>GMQSAYSFLPQVIAHRGSSGQAPENTLASLHLAGQQGIKWVEIDVMLSGDGIPVIFHDDYLSRTTDGDGLIYKTPLAELKQLDAGSWKGQEYQQETIPTLLEAIEVISQYGMGLNLELKPCEGLEEETIA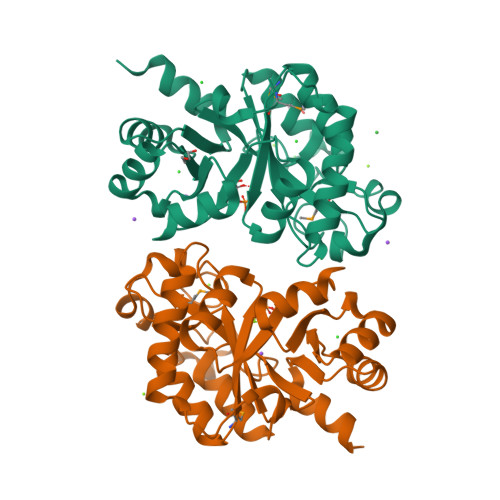ASVEVLKQHWPQDLPLLFSSFNYFALVSAKALWPEIARGYNVSAIPSAWQERLEHLDCAGLHIHQSFFDVQQVSDIKAAGYKVLAFTINDESLALKLYNQGLDAVFSDYPQKIQSAIDSHIN[4x]>PSVYDAAAQLTADVKKDLRDSWKVIGSDKKGNGVALMTTLFADNQETIGYFKRLGNVSQGMANDKLRGHSITLMYALQNFIDQLDNPDDLVCVVEKFAVNHITRKISAAEFGKFNGPIKKVLASKNFGDKYANAWAKLVAVV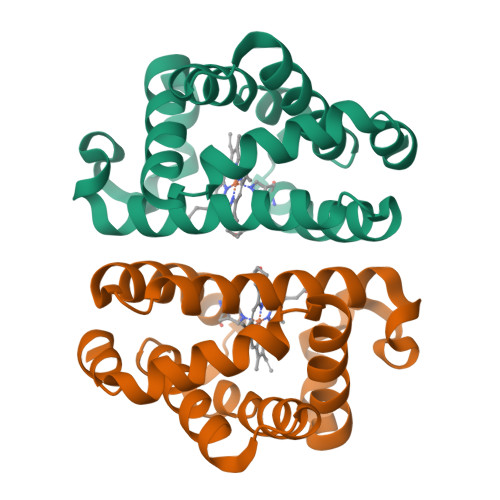QAAL[4x]(2R)-3-cyclopentyl-2-[4-(methylsulfonyl)phenyl]-N-(1,3-thiazol-2-yl)propanamide | C18 H22 N2 O3 S2 | 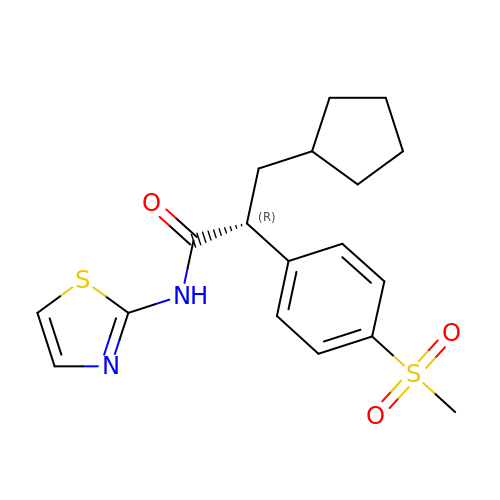NEQSWPCDHDQINX-MRXNPFEDSA-N The first step of the route is the production of N-acetyl-L-glutamate (NAG), while the second is the phosphorylation of NAG by NAG kinase (NAGK). We report here structural and functional studies on the arginine-sensitive NAGK from Saccharomyces cerevisiae (yNAGK). The structure of the mature yNAGK, lacking the N-terminal mitochondrial targeting sequence (residues 1–57), reveals an unexpected novel tetrameric architecture, which can be described as a dimer of dimers with D2 symmetry. The AAK domains occupy the center of the molecule flanked by two pairs of interacting DUF619 domains.

Although the resolution attained was 3.25 Å at the most, the high quality of the averaged electron density map allowed to unambiguously trace the entire polypeptide and to identify the majority of amino acid side chains, particularly for the DUF619 domain. The full-length enzyme tetramers consist of the AAK domains occupying the central part of the molecule, as in the truncated enzyme structure, flanked at both ends along the Q axis by a pair of interacting DUF619 domains. The central hole described for the truncated enzyme is also present, together with two narrow openings between the DUF619 and the AAK domains. The structures of the four tetramers found in the two crystals deviate from perfect D2 molecular symmetry, with three subunits in each tetramer exhibiting the open AAK domain conformation. The degree of AAK domain opening is even higher than in the arginine-containing subunit of the truncated enzyme, corresponding to a 20° rotation of the C-lobe. The pulling of the C-lobes by the paired DUF619 domains possibly contributes to this opening of the AAK domain, which is associated with rotations of up to 55° of the DUF619 domain around a hinge located at the AAK domain-DUF619 domain linker (351GYK). Comparison of the complete and truncated NAGK structures explains why the presence of the DUF619 domains does not influence the Km values for the substrates. This lack of effect on the apparent affinity for both substrates reflects the lack of physical interactions of the DUF619 domains with the substrate sites, which remain equally exposed in the structures of the truncated and the complete enzymes. The DUF619 domain is a bilobar (N-moiety, residues 354–447; C-moiety, residues 448–502) open αβα sandwich nucleated by a 7-stranded antiparallel β-sheet, which has the characteristic architecture of the histone acetyltransferase fold (GNAT fold). The comparison of the GNAT domains from NgNAGS and yNAGK (with an r.m.s.d. of 2.52 Å for 111 residues) explains why yNAGK lacks NAGS activity. The AcCoA binding site in NgNAGS, found on the boundary of the N- and C-moieties, is blocked in yNAGK (compare Figures 8E and 8F). The pairing of the DUF619 domains on each side of the yNAGK tetramer involves hydrophobic interactions between the E′ and F′ helices as well as the continuity of the central β sheets by way of antiparallel bonding of strands 6′ from both domains.

>MGHHHHHHVSSTNGFSATRSTVIQLLNNISTKREVEQYLKYFTSVSQQQFAVIKVGGAIISDNLHELASCLAFLYHVGLYPIVLHGTGPQVNGRLEAQGIEPDYIDGIRITDEHTMAVVRKCFLEQNLKLVTALEQLGVRARPITSGVFTADYLDKDKYKLVGNIKSVTKEPIEASIKAGALPILTSLAETASGQMLNVNADVAAGELARVFEPLKIVYLNEKGGIINGSTGEKISMINLDEEYDDLMKQSWVKYGTKLKIREIKELLDYLPRSSSVAIINVQDLQKELFTDSGAGTMIRRGYKLVKRSSIGEFPSADALRKALQRDAGISSGKESVASYLRYLENSDFVSYADEPLEAVAIVKKDTNVPTLDKFVCSDAAWLNNVTDNVFNVLRRDFPALQWVVSENDANIAWHFDKSQGSYLKGGKVLFWYGIDDINTISELVENFVKSCDTASTLNSSASS[8x]(1S,3R,5Z,7E,14beta,17alpha,20S)-20-(3-hydroxy-3-methylbutoxy)-9,10-secopregna-5,7,10-triene-1,3-diol 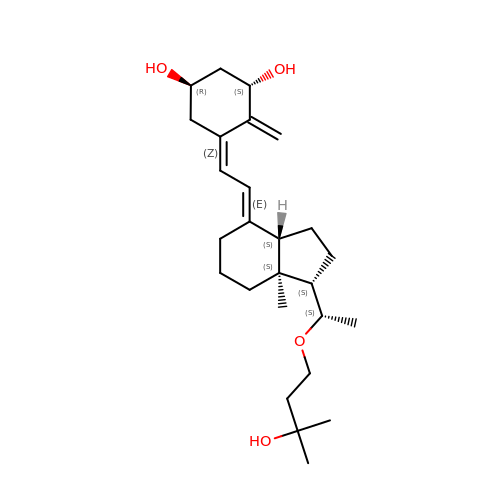| C26 H42 O4 | DTXXSJZBSTYZKE-ZDQKKZTESA-N> SEGNGPAAVHYQPASPPRDACVYSSCYCEENVWKLC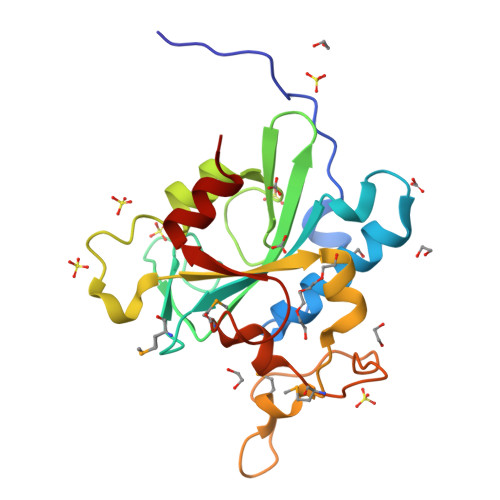EYIKNHDQYPLEECYAVFISNERKMIPIWKQQARPGDGPVIWDYHVVLLHVSSGGQSFIYDLDTVLPFPCLFDTYVEDAIKSDDDIHPQFRRKFRVICADSYLKNFASDRSHMKDSSGNWREPPPPYPCIETGDSKMNLNDFISMDPKVGWGAVYTLSEFTHRFGS> SEICPSFQRVIE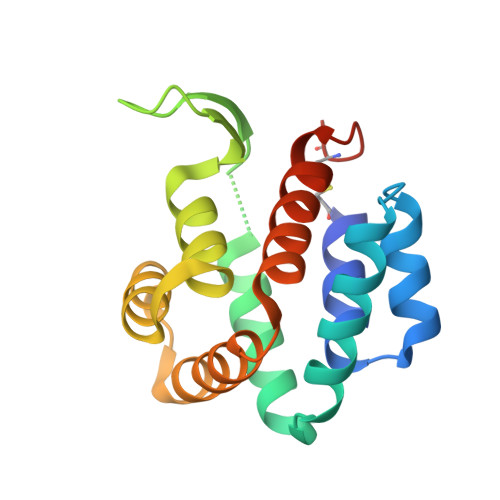TLLMDTPSSYEAAMELFSPDQDMREAGAQLKKLVDTLPQKPRESIIKLMEKIAQSSLSGWRPYIERWTGRLIVGSPSFQRVIETLLMDTPSSYEAAMELFSPDQDMREAGAQLKKLVDTLPQKPRESIIKLMEKIAQSSLCNHHHHHH> HHHHHHSSGLVPRGSHMKTTTQELKQYM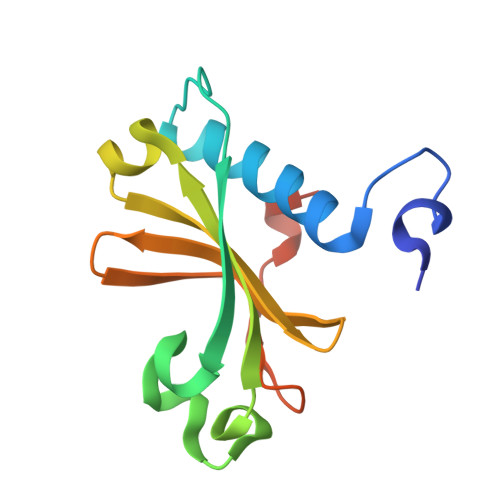TRLFQLSNNETWECETLEEAAENILPKRFINDSPLAHLILETYTYYNNELHELSIYPFLMYSNNQLISIGYLDHFDMDFLYLTDTKNTIIDERHLLKEGGNNHE>MWFGEFGGQYVPETLVGPLKELEKAYKRFKDDEEFNRQLNYYLKTWAGRPTPLYYAKRLTEKIGGAKVYLKREDLVHGGAHKTNNAIGQALLAKLMGKTRLIAETGAGQHGVATAMAGALLGMKVDIYMGAEDVERQKMNVFRMKLLGANVIPVNSGSRTLKDAINEALRDWVATFEYTHYLIGSVVGPHPYPTIVRDFQSVIGREAKAQILEAEGQLPDVIVACVGGGSNAMGIFYPFVNDKKVKLVGVEAGGKGLESGKHSASLNAGQVGVSEGMLSYFLQDEEGQIKPSHSIAPGLDYPGVGPEHAYLKKIQRAEYVAVTDEEALKAFHELSRTEGIIPALESAHAVAYAMKLAKEMSRDEIIIVNLSGRGDKDLDIVLKASGNVLEHHHHHH[4x]

The second enzyme we screen is a previously-engineered β-subunit of tryptophan synthase from the thermophilic archaeon Pyrococcus furiosus (PfTrpB2B9, or 2B9), which catalyzes the bimolecular condensation of Ser and indole. It has been demonstrated that 2B9 possesses a broad substrate scope, and is capable of producing diverse Trp analogs. We hypothesized that a different mutation at H275 might increase activity, rather than reduce it. This hypothesis was further motivated by the location of H275, which is a ‘second-sphere’ residue situated near the entrance to the enzyme’s active site. We also observed mutations that resulted in a general increase in activity across all substrates screened, with H275E displaying the largest boost.

To determine how products fit within the active site, we solved the structure of H275E with two ligands bound, Trp and 4-Cl-Trp, at 2.39 and 2.25-Å resolution, respectively. The structure of H275E with 4-Cl-Trp bound showed no major conformational change is required to accommodate the 4-Cl group. Instead, there is a 3.0-Å halogen bond to G298. We subsequently validated that H275E has increased activity in single substrate reactions, and these improvements extend to substrates that were not present in the original screen, such as the sterically bulky nucleophile 5-OEt-indole.> SVHVPGPHAMTIQELVDYVNARQKQGIYEEYEDIRRENPVGTFHCSMSPGNLEKNRYGDVPCLDQTRVKLTKRSGHTQTDYINASFMDGYKQKNAYIGTQG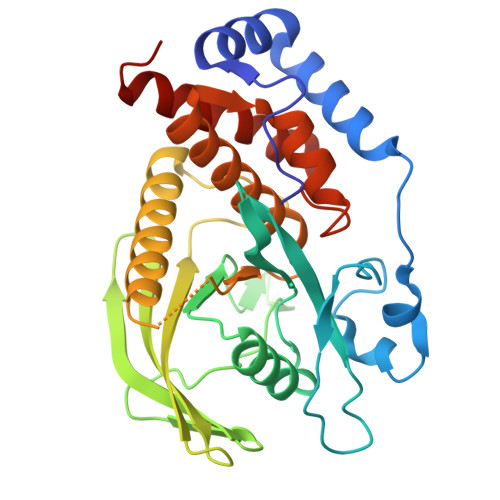PLENTYRDFWLMVWEQKVLVIVMTTRFEEGGRRKCGQYWPLEKDSRIRFGFLTVTNLGVENMNHYKKTTLEIHNTEERQKRQVTHFQFLSWPAYGVPSSAASLIDFLRVVRNQQSLAVSNMGARSKGQCPEPPIVVHASAGIGRTGTFCSLDICLAQLEELGTLNVFQTVSRMRTQRAFSIQTPEQYYFCYKAILEFAEKEGMVSS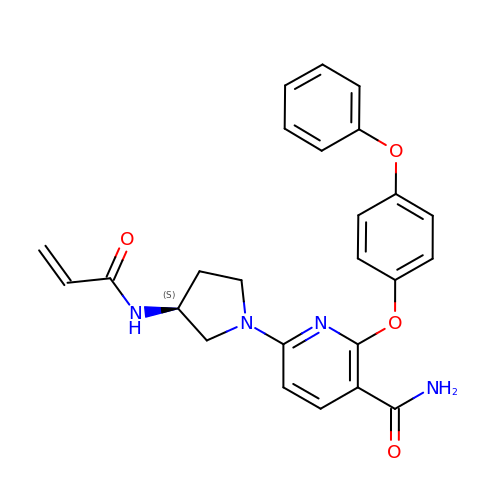6-[(3S)-3-(acryloylamino)pyrrolidin-1-yl]-2-(4-phenoxyphenoxy)pyridine-3-carboxamide | C25 H24 N4 O4 | VMINNJIVIPLCSD-KRWDZBQOSA-N> ICVNENGGCEQYCSDHTGTKRSCRCHEGYSLLADGVSCTPTVEYPCGKI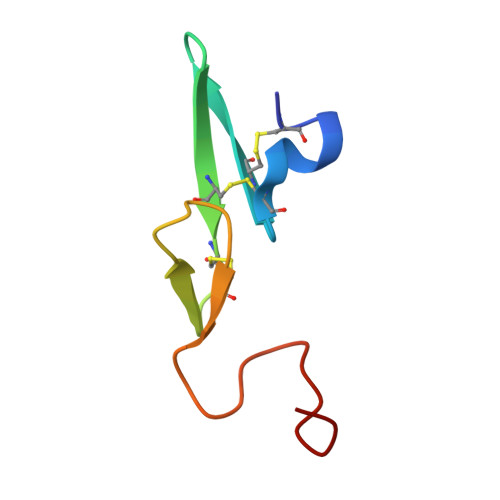PILE> SMAAQKNNAPKEYGADSITILEGLEAVRKRPGMYIGSTGERGLHHLIWEVVDNAVDEAMAGFATRVD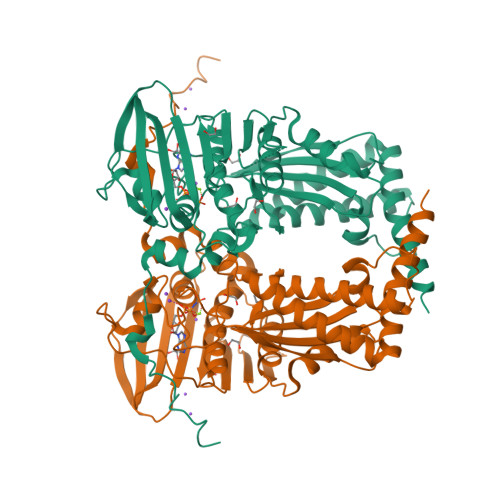VKIHADGSVEVRDDGRGIPVEMHATGMPTIDVVMTQLHAGGKFDGETYAVSGGLHGVGVSVVNALSTRLEATVLRDGYEWFQYYDRSVPGKLKQGGETKETGTTIRFWADPEIFETTDYNFETVARRLQEMAFLNKGLTIELTDERVTAEEVVDDVVKDTAEAPKTADEKAAEATGPSKVKHRVFHYPGGLVDYVKHINRTKTPIQQSIIDFDGKGPGHEVEIAMQWNAGYSESVHTFANTINTHEGGTHEEGFRAALTSVVNRYAKDKKLLKDKDPNLTGDDIREGLAAVISVKVAEPQFEGQTKTKLGNTEVKSFVQKICNEQLQHWFEANPAEAKTVVNKAVSSAQARIAARKARELV> ISVRGLAGVENVTELKKNFNRHLHFTLVKDRNVATPRDYYFALAHTVRDHLVGRWIRTQQHYYEKDPKRIYYLSLEFYMGRTLQNTMVNLALENACDEATYQLGLDMEELEEIEEDAGLGNGGLGRLAACFLDSMATLGLAAYGYGIRYEFGIFNQKICGGWQMEEADDWLRYGNPWEKARPEFTLPVHFYGRVEHTSQGAKWVDTQVVLAMPYDTPVPGYRNNVVNTMRLWSAKAPNDFNLKDFNVGGYIQAVLDRNLAENISRVLYPNDNFFEGKELRLKQEYFVVAATLQDIIRRFKSSKFGCRDPVRTNFDAFPDKVAIQLNDTHPSLAIPELMRVLVDLERLDWDKAWEVTVKTCAYTNHTVIPEALERWPVHLLETLLPRHLQIIYEINQRFLNRVAAAFPGDVDRLRRMSLVEEGAVKRINMAHLCIAGS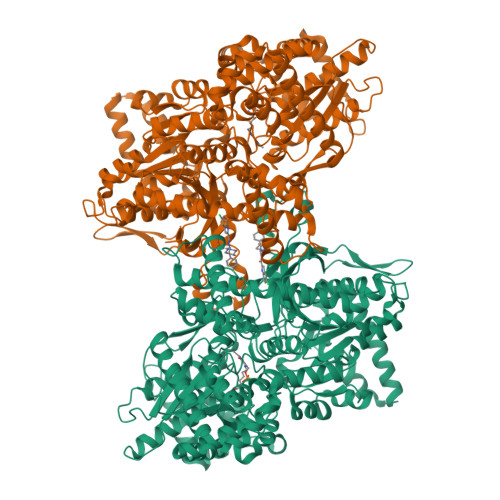HAVNGVARIHSEILKKTIFKDFYELEPHKFQNKTNGITPRRWLVLCNPGLAEIIAERIGEEYISDLDQLRKLLSYVDDEAFIRDVAKVKQENKLKFAAYLEREYKVHINPNSLFDVQVKRIHEYKRQLLNCLHVITLYNRIKKEPNKFVVPRTVMIGGKAAPGYHMAKMIIKLITAIGDVVNHDPVVGDRLRVIFLENYRVSLAEKVIPAADLSEQISTAGTEASGTGNMKFMLNGALTIGTMDGANVEMAEEAGEENFFIFGMRVEDVDRLDQRGYNAQEYYDRIPELRQIIEQLSSGFFSPKQPDLFKDIVNMLMHHDRFKVFADYEEYVKCQERVSALYKNPREWTRMVIRNIATSGKFSSDRTIAQYAREIWGVEPSRQRLPAPDEKIP Glucoamylases (GA: EC 3.2.1.3, 1,4-α-D-glucan glucohydrolase) are amylolytic enzymes, possessing specific raw starch-binding ability through their carbohydrate-binding module (CBMs). GAs from Rhizopus oryzae (RoGA) posses an N-terminal starch binding domain (SBD), which belongs to CBM family 21 (RoCBM21) and shares relatively low level similarity with the SBDs derived from other starch-processing enzymes. RoCBM21 has been proposed to have a cooperative mode of interaction to sugar molecules, which are dominated by hydrophobic-binding region created by aromatic residues namely Trp47, Tyr83, and Tyr94 at site I and Tyr32 and Phe58 at site II. We previously created a circularly permuted form of RoCBM21 in which the original N and C termini of RoCBM21 were joined and new termini were created at positions 89 and 90.

Unlike most other constructed circularly permutated proteins, CP90 had significantly enhanced binding affinity and improved selectivity toward long-chain carbohydrates (i.e., its affinity for β-cyclodextrin is less than that for amylose EX-I, which is less than that for soluble and insoluble starches). The asymmetric unit of CP90 reveals a homodimer in which each unit is arranged in a slightly tilted antiparallel fashion. The RoCBM21 and the CP90 share a similar overall topology. CP90 crystal structure showed only 7 β-sheets while RoCBM21 has 8 β-sheets. The major interface contacts involve hydrophobic and hydrogen bond interactions, which were mapped onto the CP90 structure using Pymol. The super-positioning of RoCBM21 and CP90 showed that substantial shift in the orientation of amino acids either at site I or site II had not occurred. However, two of the aromatic residues (Tyr93 and Tyr94) and one hydrophilic residue (Asn101), which form part of binding pocket in the RoCBM21 have been moved to the N-terminal unstructured region in CP90 (see the unstructured region in Figure 1). The dominant negative charge near the binding site II is caused by the replacement of positively charged Lys91 in RoCBM21 to the N-terminal unstructured region of CP90 and the additional negative charge provided by the C-terminal carboxyl, which is proximal to the site II of CP90. Although CP90 can adopt the second binding path (hydrophilic binding path), the dimerisation provides an alternate binding path to connect the binding site I and II. The proposed alternate binding path for CP90 involves the hydrophilic residues Lys54, Lys55, Glu107 near the binding site residue Tyr52 in one subunit that connect to the next subunit through hydrophilic core Lys97, Asp62, Asp65, Asp68, Asn69, Asn70 and Asn72 situated near second binding site residue Trp67.

>MGKTYYDNNNSANYQVSTHMASIPSSASVQLDSYNYDGSTFSGKIYVKNIAYSKKVTVVYADGSDNWNNNGNIIAASFSGPISGSNYEYWTFSASVKGIKEFYIKYEVS[2x]> MIKQRTLKRIVQATGVGLHTGKKVTLTLRPAPANTGVIYRRTDLNPPVDFPADAKSVRDTMLCTCLVNEHDVRISTVEHLNAALAGLGIDNIV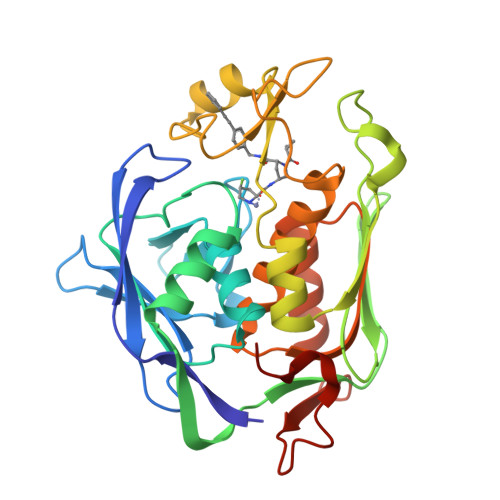IEVNAPEIPIMDGSAAPFVYLLLDAGIDELNCAKKFVRIKETVRVEDGDKWAEFKPYNGFSLDFTIDFNHPAIDSSNQRYAMNFSADAFMRQISRARTFGFMRDIEYLQSRGLCLGGSFDCAIVVDDYRVLNEDGLRFEDEFVRHKMLDAIGDLFMCGHNIIGAFTAYKSGHALNNKLLQAVLAKQEAWEYVTFQDDAELPLAFKAPSAVLA> GSDQEAKPSTEDLGDKKE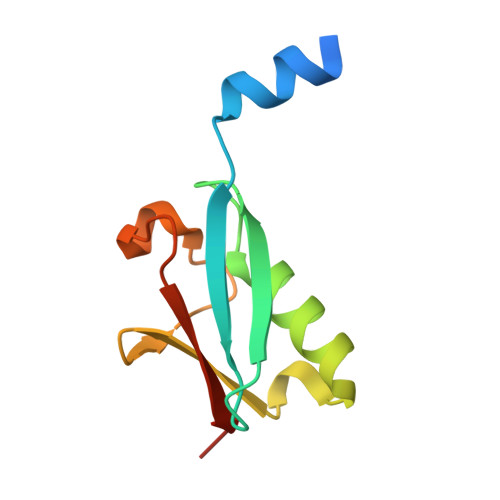GEYIKLKVIGQDSSEIHFKVKMTTHLKKLKESYAQRQGVPMNSLRFLFEGQRIADNHTPKELGMEEEDVIEVYQEQTGG> MGHHHHHHHHHHEPPAIPHITEGFYPLPEIVETFSHHVLQELVSLAEVLPSMSNVEKKKKILDWLLRSRAFTMRLLVLARWVHLSPSVHRCIDVVAFLQGQKFCFQNLVHVLQDIRYQLSFARLRNSDLVTALDILSTGTSLRLANAPTSKLYMLSESPLSTKQILQTLHALNMLIRIRLSLYEIIPTPFQHFTIANGRCTFTVPNEFSVSLTTNSQDPKSTGISFQWIVVDFQFHLPDFSSTPAKYRVFIELHLNEEIAAAFVLQKPILPLIYNILHKFCLYQRLNLLSQQTFQLSRESWLGHLRGVYDEKPPRLRLYYWPQLNVKKEGKPGKIGHYIHIFVNTQPISAFERTLSSKRSSCEYDHFLLLVEWHHDGIVEHVPLDDHMDAQHLLLLITQKHAQLILEQIRKELHPNIFSEHVGGGLK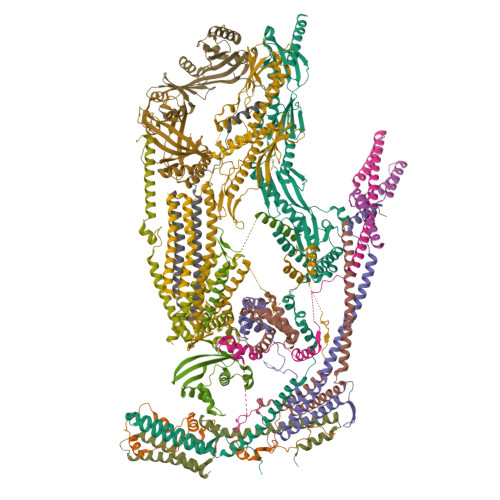IHVFDNEIIVKVNSVTGRLVLSSSASPLSPPRHLRAAEKNIALNTQPPAQILNRLYFFCIQTQLLEVAQCAELHAVQGYYSFPYLTFSKGKWRKDGDSLWVLAYNVESNSWSVRLLNAAGQTLYTQDVHTTKGTLSIESFSRLSYLLEVQILLFNVQTACQARG;> MLPQDDMTDEMKSLASRLEDTTQAFYDLALIVYNLEDTTPSDAIPESLDTLIRDLKSLPDISRKVNNLIPQDVLEYIEQGRNPDVYARQFSELVQKDNQYVNGKLYAIEGFQKAFAEEIKQAYPEVSSVVDKILNEGKVESTVS;> MAQAPEYHYVGSVDYQPTRPSAHQNLIELYGLTELAKKVGRVDEFGNKRKMRRSYKAYIQDLPGYNEILRDNTIKQWLTNPIREEVPIDIEFLHHVFSVEPGIIPGFNPKVFGLEDDVVMGNVSRDSSQPRSPSRRKK;> MACRCTQLQDTIDEVATQFYSSIHYLSSHHDFVPLPGQEKVSDSKVNPISAEELQFAQRDLAKDLVTKFMQIDTLINQLPGISTAPKHQLEKIKKLQNSIEEKQLERKSLESENEDLKLQLAKRIETFGRLSCVLFQP;> MEPNEGVQLFSAFPPPPPYYKLFTRENIEKVISNMEKEAKHEDDANTLQPKTEEEIESLAKLFKKPSCLTSGTYQMFGDTWRLDEAIPSLKEFGIPELYKDIKDGEDEIEVVEYDPKSNAIVGTSFTRVHDYDKNSPIENEKILEDDQHTAMKEKDNESDKTMKDVEEKTEPSLKKEEEDIQMKEPLDSQDTGAVSASSVNEGFRADQKSKDGETSDLIKIPRRAYELRFLSRSLMLNFLELLGIMAKAPEQFPSKVENIRVLLLNLHHLINDYRPHQSRESLIMLLEKQLKHEESQVELLRTHNRQMTETLEKYKSLDFNMEKEGDVIQQLKSSIKKPLSGAEDEQKSRSMFSKNDEKLKKSLELMEDVIKRDLS;> MDPAHHIKDTSAELLSQQDFSILQSRLLEFLASQEARETVTASKELTLLRQGIRQLKEKVSKMEPEEMTVKEKKSIIEILKARIALKKAFLKMALSESNDTVVKKEDVRESPVDTFMENAT;> MEYQRAIDSIEECLNKQLRLSSEKVDQYVLIENWTSLVGHLKTLHSLISNYTNGRELQNEISSLLKQDKELDLQIQDCMREMTSIYDTHLPKTVSGRKRQKVNAETLLDYGRKLSKFSSAPPGYNPETGQDAKAPVHYPWPSEDQMRKTLLFQFSTSMVPNLSATASQLFSEQPPKTNEPTETETEIDANKAVEEKTKMNYPASPTFTTQEENKEVESPANKDVFAGFDLFDPEMEEDF;> METKWLLSKVPDDKSRFEIELEFVQMLSNPWYLNFLAQHKYFEDEAFLQYLEYMEYWREPEYVKFIIYPTCLHMLTLLKNPQFRNDISRADLSKQVNDEIYYEWLGKGLQQYGSADDATLSQPQQEEDEKKVDVKKENE;> MASGAPPSVDLTSIQWRMPEWVQSMGGLRTENVLEYFSQSPFYSHKSNNEMLKMQSQFNALDLGDLNSQLKRLTGIQFVIIHERPPFLWVIQKQNRLNENEVKPLTVYFVCNENIYMAPNAYTLLATRMLNATYCFQKALTKIEKFPQYNPQEGYTYPKLSNDNLEVDHSNTNEPADENKNQSIENADYSFSPEDFSVVRAFMQSLHSSKEAPDVK;> MEDISTEKTVESLEAIRHRIAQIVQSLTHFLAILHQSESLSPWPTIHKNFNILLSQIHSLSNNLAAHSHTLQTTSIYPSLEFPVKEQEPLLTTLLRTKALPEVEEWEANTLQEYEASISSQPKKKEANDAYQKDQLWDQARIIFMEERENYSWFDFVTRRQESEGEFVSQRQLEIDRATEEQNANQMLTDILSFMKSGKR;> MTNSDDDLFSEKSTSSDTQQVQNILELEAKIPDILSSAGKCIEAIQLNNSLEDFRKYSKEFLETVEFISTGLRRQALELEKAEVPVVSLQPKKRYASTPLSNLIFDQSSKLM;> MAEEANKDADISSLSLSLDPEIIGGQNNFLENNLQQIFQKIIQERGPFRDLKEEDLQKELQKESIKDESSAKSSETENVLEFATLDSKRNVNDTEVESMDSQAYKKELIEQIMIAQTECSLALDMTSLLLSKFKENSIETISPFLKSTVPPSSLQFSRSQPPESKESDATLAKCWKEKSLTSSCKFLFEAKERLTSVVETEHEYYTELVKVKEASWPLFNSQGSNHLSVQYSCLGGISLGLGLIRMKPESKSFEVQSSLLYSQAALKISILNKDRDEIGSSTWSWPSQNCNSVLLKDIYKLQEILFEMDIWNSLLQEAQSCGNQGVNFTGDEILVPISDDHVVRITLETSSKNTESGFTEDKKSNEDTSTNFVTIKQEKELLKCLCDTLNAIAHILFLKHCRKSDRRSQQPELYMAIDANAPLILRPLIFYYNLNQESLEFQRWLKQRDISFKFMPNYPWEKAKDFLELENSLSINRLSISWRIMVSNFEPAIFIQHTPTLHGTDKSVWRCKDQYSSNQFSSLKNVCQYIEHHINSLSRRSKKTE;> MASMQELYLLGVVPSRRFEAVVNSLSKTLDGPKTILEFWVVYRPKDVPPNLPRQPDSWLRLCSNIESHDETDTEWSKNTQWSMYLEGNSEPKREDKCGIRPVNRAKLTNGSVTEFVEKMGYEFSHEYIIQGLEYFFFDTTVRIYQTLIPSQQRSIKPPFHPMNEEQPWILHVYTHVADASNQVAMAKAEANLTKVKTLLSAFCDLKNVRL;> MPVHGVIYYSSPSMATFLSPAQDNLVRTYFAQHLKKWVVQYKLYRNAVTPKTLEFLKQNINPSMLACVDEATMIDAEPELEDIIVRTKLWNFRQSFTIEGSIYEVGSFKVAIANVLQKSVWKGILFHVTYDGTESVDLARPIIQEFFLKCFLQNNKSVTPVYESFFNQPRHSLDSKLLLQLFKQRIDTVSQRT;> MSSDSFQRQLVQRTNTLNSSIDNATLTILSRFQDILDIAINEGKDKYTVAPEVYQIECHTVSMVRAVEQLLDVSRQIKSYWLTNSLSTSFPTVDYSEPDLEKVKRTLTKLQNHLLEVSLIEPEASETTEAPTVSDT(2E)-3-[(7R)-7-amino-8-oxo-6,7,8,9-tetrahydro-5H-pyrido[2,3-b]azepin-3-yl]-N-methyl-N-[(3-methyl-1-benzofuran-2-yl)methyl]prop-2-enamide | C23 H24 N4 O3 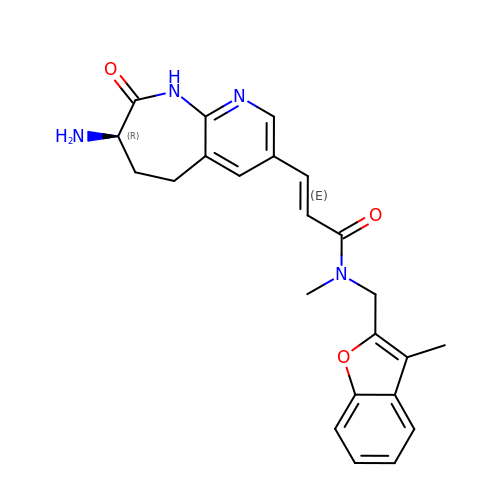| ZWQNEFFHBSGFHV-RUJXFNLJSA-N> AVTLDKDAYYRRVKRLYSNWRKGEDEYANVDAIVVSVGVDEEIVYAKSTALQTWLFGYELTDTIMVFCDDKIIFMASKKKVEFLKQIANTKGNENANGAPAITLLIREKNESNKSSFDKMIEAIKESKNGKKIGVFSKDKFPGEFMKSWNDCLNKEGFDKIDISAVVAYTIAVKEDGELNLMKKAASITSEVFNKFFKERVMEIVDADEKVRHSKLAESVEKAIEEKKYLAGADPSTVEMCYPPIIQSGGNYNLKFSVVSDKNHMHFGAITCAMGIRFKSYCSNLVRTLMVDPSQEVQENYNFLLQLQEELLKELRHGVKICDVYNAVMDVVKKQKPELLNKITK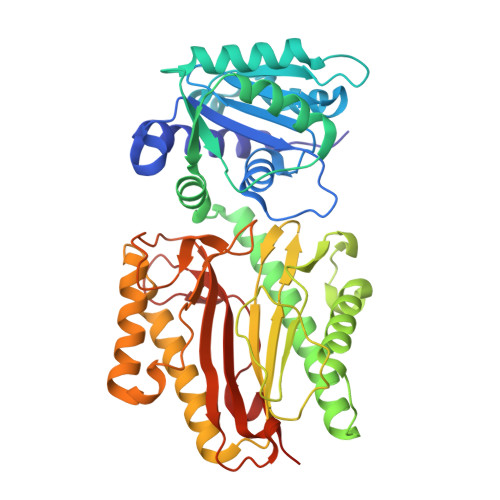NLGFGMGIEFREGSLVINSKNQYKLKKGMVFSINLGFSDLTNKEGKKPEEKTYALFIGDTVLVDEDGPATVLTSVKKKVKNVGIFL> ASPSSELRRALEANEFIPYYQPLSPGQGGRWIGVEVLMRWRHPREGLIRPDLFIPFAERSGLIVPMTRALMRQVAEDLGGHAGKLEPGFHIGFNISATHCHELALVDDCRELLAAFPPGHITLVLELTERELIESSEVTDRLFDELHALGVKIAIDDFGTGHSSLAYLRKFQVDCLKIDQSFVARIGIDTLSGHI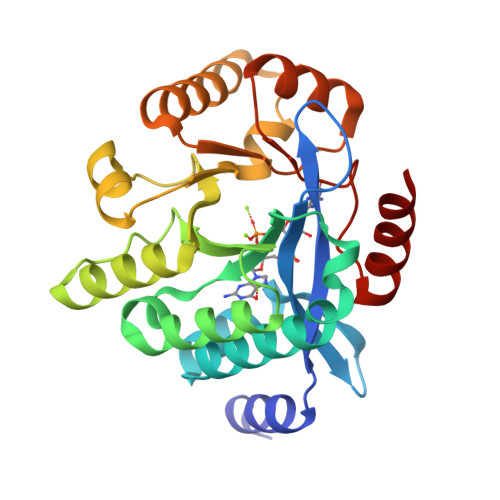LDSIVELSAKLDLDIVAEGVETPEQRDYLAARGVDYLQGYLIGRPMPLESLLSSLTVQEQQ> GDRVADMIESSIGDSVSRALTQALPAPTGQNTQVSSHRLDTGEVPALQAAEIGASSNTSDESMIETRCVLNSHSTAETTLDSFFSRAGLVGEIDLPLEGTTNPSGYANWDIDITGYAQMRRKVELFTYMRFDAEFTFVACTPTGQVVPQLLQYM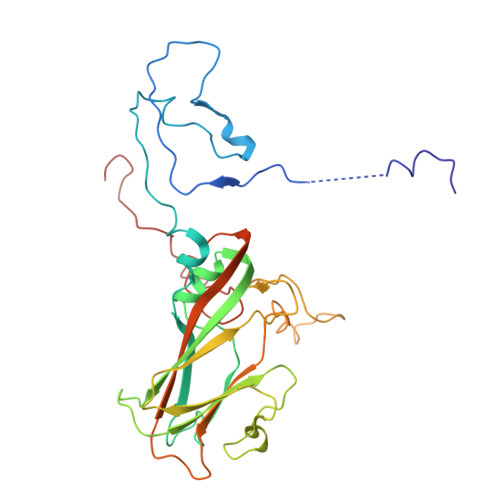FVPPGAPKPESRESLAWQTATNPSVFVKLTDPPAQVSVPFMSPASAYQWFYDGYPTFGEHKQEKDLEYGACPNNMMGTFSVRTVGSSKSKYALVVRIYMRMKHVRAWIPRPMRNQNYLFKANPNYAGDSIKPTGTSRNAITTL> MIDKSIMKKLLLTFLSIAAVCSLYAQRKVTQERMEQIYEEVKTPYKYGLAVAPTDNYHKIDCPTVFRQGDKWLMTYVVYNGKTGTDGRGYETWIAESDNLLDWRTLGRVLSYRDGKWDCNQRGGFPALPDMEWGGSYELQTYKGRHWMTYIGGEGTGYEAVKAPLFVGLASTKGDISTAHEWESLDKPILSIHDKDAQWWEKLTQYKSTVYWDKDKTLGAPFVMFYNAGGRHPE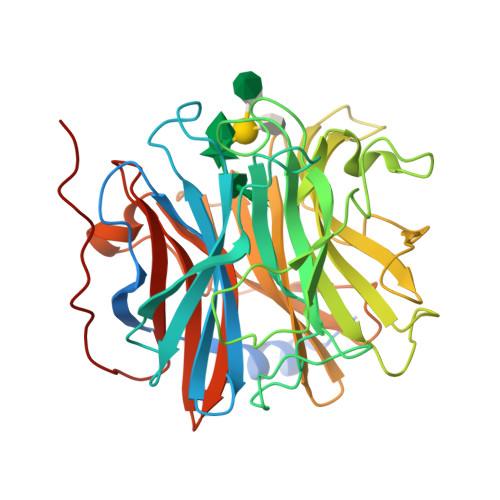TDLKGQRVGIALSKDMKTWKRYPGNPVFAHEADGTITGDAHIQKMGDVYVMFYFSAFEPSRKYKAFNTFAASYDLVNWTDWHGADLIIPSKNYDELFAHKSYVIKHDGVVYHFYCAVNNAEQRGIAIATSKPMGRSAVRFPKPETKN>TRDFNGTWEMESNENFEGYMKALDIDFATRKIAVRLTFTDVIDQDGDNFKTKATSTFLNYDEDFTVGVEFDEYTKSLDNRHVKALVTWEGDVLVCVQKGEKENRGWKKWIEGDKLYLELTCGDQVCRQVFKKK[3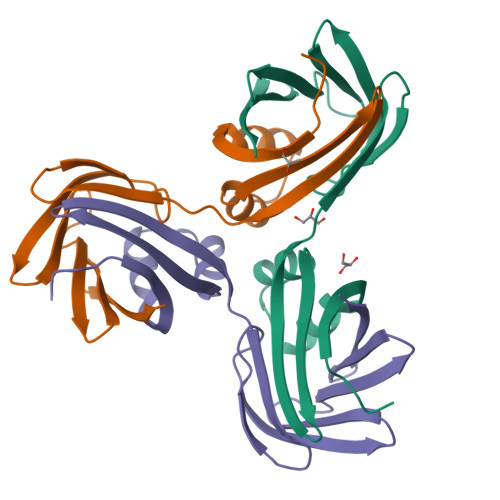x]>[2x]SEFLSSEVITQVRSLLNQGYRI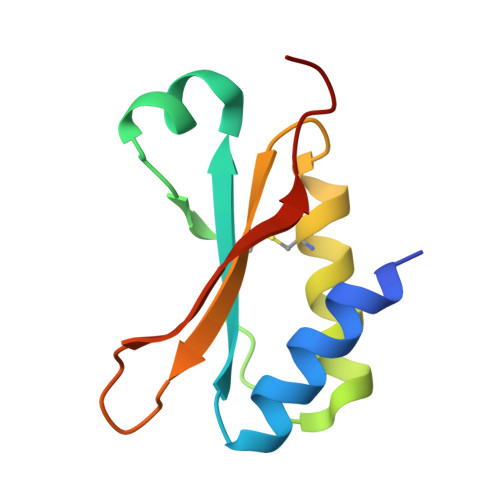GTEHADKRRFRTSSWQPCAPIQSTNERQVLSELENCLSEHEGEYVRLLGIDTNTRSRVFEALIQRPDGSV>MGSMYVVGHKIPDSDSICGAIALAYLKNQIGEPAIAARLGELSPETAFILEKFGFEAPEYKTSYAGEEVYIVDH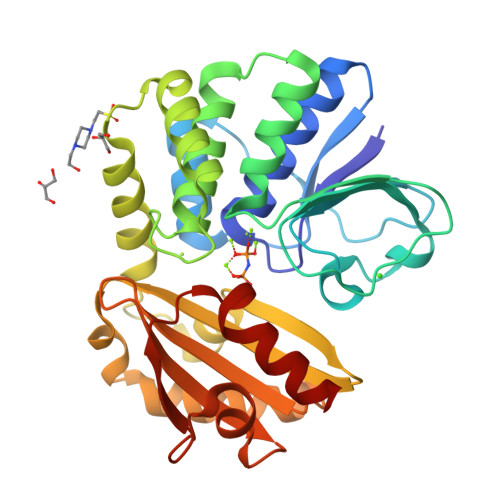SEITQAPDDIAQATIVGIVDHHKLGDLTTSTPLECWIRPVGCSNTVIKMMYDFYQVKIPANIAGIMMCAILSDTVIFKSPTCTTADIRCVEALAEIAGVEDFKEVGMDMFKVKSAVEGTPARDLVMRDFKDFNMNGNLVGIGQLEVIDLAVFDDIKADLEADIAKLKVEGNRHSVLLLLTDIMKEGSEMLVVSDSADLTERAYGKPTVDGRVWLDGVLSRKKQVVPALQDAFQKV[2x]> TQDLNFGQVVADVLCEFLEVAVHLILYVREVYPVGIFQKR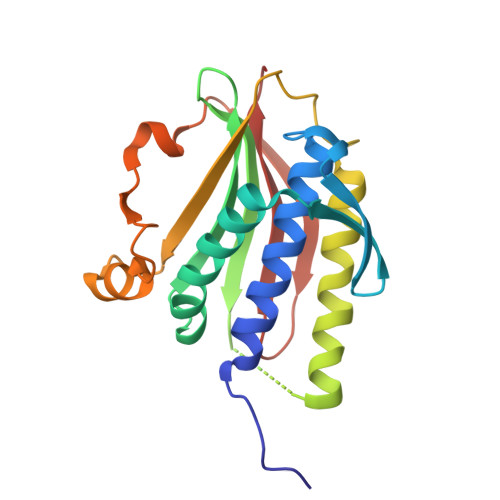KKYNVPVQMSCHPELNQYIQDTLHCVKPLLEKNDVEKVVVVILDKEHRPVEKFVFEITQPPLLSISSDSLLSHVEQLLRAFILKISVCDAVLDHNPPGCTFTVLVHTREAATRNMEKIQVIKDFPWILADEQDVHMHDPRLIPLKTMTSDILKMQLYVEERAHK> MIPT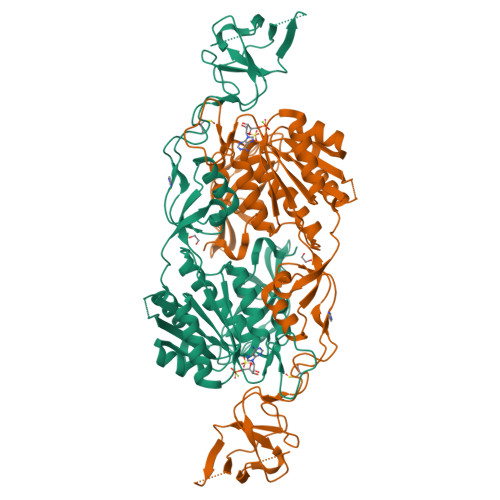EEALRIVFGVSKRLPPVIVSLYEALGKVLAEDIRAPDPLPPYPASVKDGYAVVASDGPGEYPVITESRAGNDGLGVTVTPGTVAYVTTGGPIPDGADAVVQVEDTKVIGDVSTESKRVKILIQTKKGTDIRRVGCDIEKDATVLTTGERIGASEIGLLATAGVTMVKVYPMPIVAILSTGDELVEPTAGTLGRGQIRDSNRAMLVAAVMQQQCKVVDLGIVRDDRKELEKVLDEAVSSGVDIILTSGGVSMGDRDFVKPLLEEKGKVYFSKVLMKPGKPLTFAEIRAKPTESMLGKTVLAFGLPGNPVSCLVCFNIFVVPTIRQLAGWTSPHPLRVRLRLQEPIKSDPIRPEFHRAIIKWKDNDGSGTPGFVAESTGHQMSSRLLSMRSANALLELPATGNVLSAGSSVSAIIVSDISAFSID> MNARSTGQHPARYPGAAAGEPTLDSWQEPPHNRWAFAHLGEMVPSAAVSRRPVNAPGHALARLGAIAAQLPDLEQRLEQTYTDAFLVLRGTEVVAEYYRAGFAPDDRHLLMAVSKSLCGTVVGALVDEGRIDPAQPVTEYVPELAGSVYDGPSVLQVLDMQISIDYNEDYVDPASEVQTHDRSAGWATRRHGDPADTYEFLTTLRGDGSTGEFQYCSANTDVLAWIVERVTGLRYVEALSTYLWAKLDADRDATITVDTTGFGFANGGVSCTARDLARVG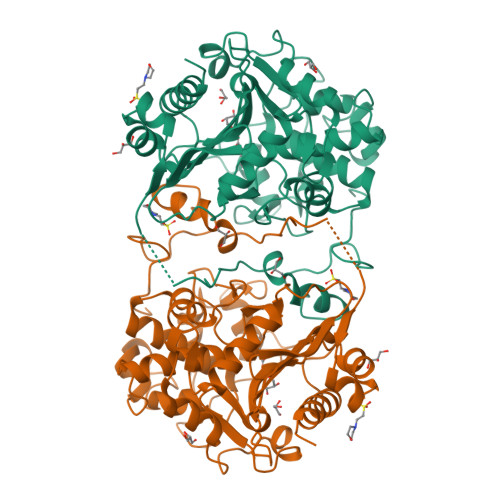RMMLDGGVAPGGRVVSEDWVRRVLAGGSHEAMTDKGFTNTFPDGSYTRQWWCTGNERGNVSGIGIHGQNLWLDPLTDSVIVKLSSWPDPYTEHWHRLQNGILLDVSRALDAV{2-[(1-benzofuran-2-ylmethoxy)carbonyl]-5-methoxy-1H-indol-1-yl}acetic acid 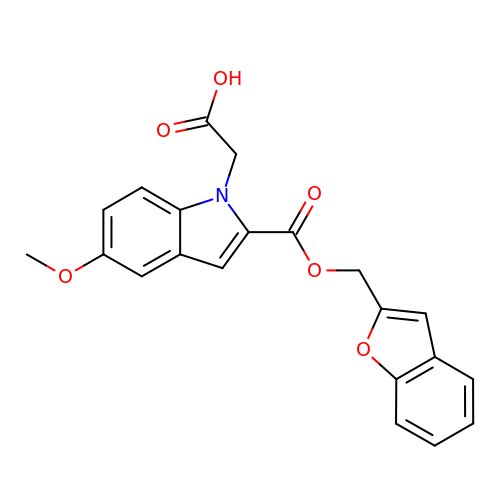| C21 H17 N O6 | CKGFVKXFHXZPEW-UHFFFAOYSA-N4-[(Z)-1-cyano-2-{6-[(2-hydroxyethyl)(methyl)amino]-1-benzothiophen-2-yl}ethenyl]benzonitrile | C21 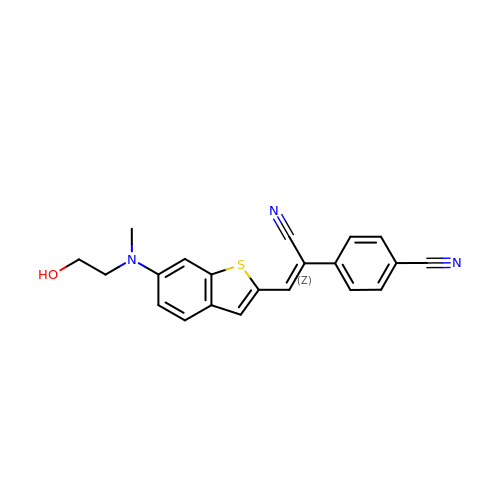H17 N3 O S | WXTHEUULEXARCU-WOJGMQOQSA-N> GHMLQNNTDYPFEANNPYMYHENPMEEGLSMLKLANLAEAALAFEAVCQAAPEREEAWRSLGLTQAENEKDGLAIIALNHARMLDPKDIAVHAALAVSHTNEHNANAALASLRAWLLSQPQYEQLGSVNLQADVDIDDLNVQSEDFFFAAPNEYRECRTLLHAALEMNPNDAQLHASLGVLYNLSNNYDSAAANLRRAVELRPDDAQLWNKLGATLANGNRPQEAL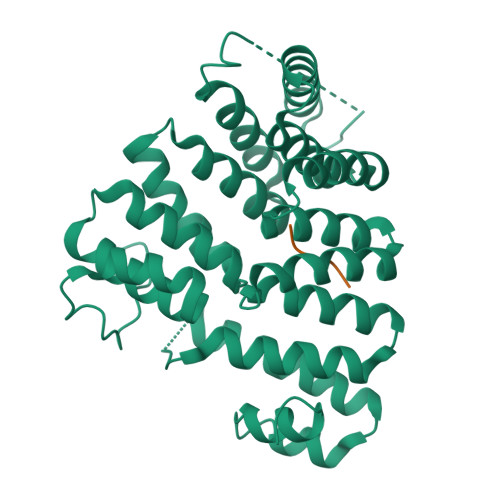DAYNRALDINPGYVRVMYNMAVSYSNMSQYDLAAKQLVRAIYMQVGGTTPTGEASREATRSMWDFFRMLLNVMNRPDLVELTYAQNVEPFAKEFGLQSMLL;> HEELAKL> 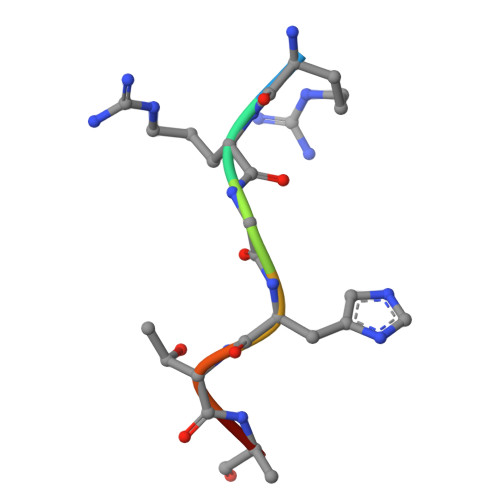RRGHTAS> GAACGACAGTGA;> CGTCGACTC;> TCAACG;> TC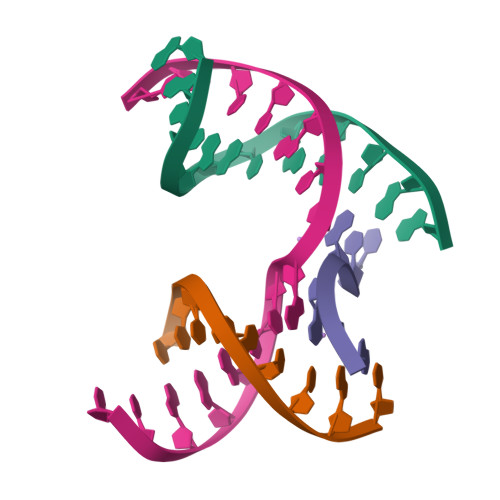GAGTCGCTGTCGT(2R)-5-(acetyloxymethyl)-2-[(1R)-1-[[(5R)-5-azanyl-6-oxidanyl-6-oxidanylidene-hexanoyl]amino]-2-oxidanylidene-ethyl]-5,6-dihydro-2H-1,3-thiazine-4-carboxylic 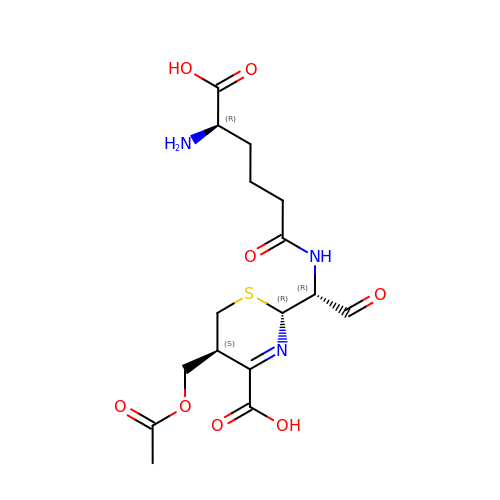acid | C16 H23 N3 O8 S | KPDUYBJZYVMEKK-ICUOPCATSA-N>SNAMKLINTTWTHQELVNNQLDNTDAFLVETYSAGNTDVVFTQAPKHYELLISNKHRAVKDNELEVIREFFLKRKIDKDIVLMDKLRTVHTDKL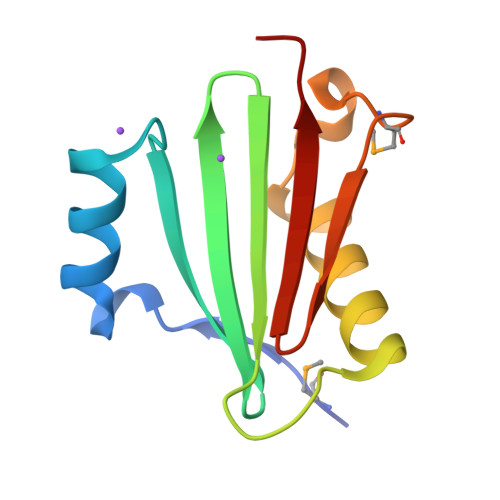IEISFPTTV[4x]>[2x]HHLFKEAQAFIENMYKECHYETQIINKRLHDIELEIKETGTYTHTEEELIYGAKMAWRNSNRCIGRLFWDSLNVIDARDVTDEASFLSSITYHITQATNEGKLKPYITIYAPKDGPKIFNNQLIRYAGYDNCGDPAEKEVTRLANHLGWKGKGTNFDVLPLIYQLPNESVKFYEYPTSLIKEVPIEHNHYPKLRKLNLKWYAVPIISNMDLKIGGIVYPTAPFNGWYMVTEIGVRNFI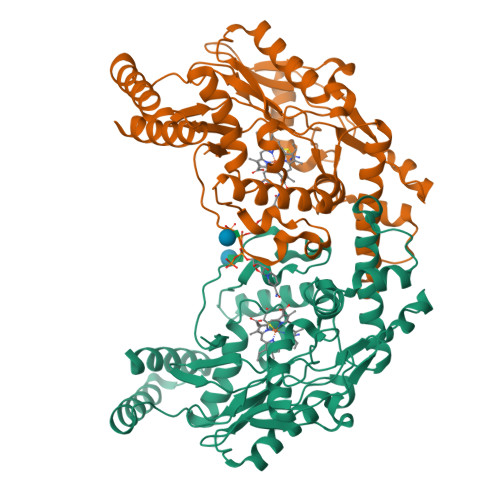DDYRYNLLEKVADAFEFDTLKNNSFNKDRALVELNYAVYHSFKKEGVSIVDHLTAAKQFELFERNEAQQGRQVTGKWSWLAPPLSPTLTSNYHHGYDNTVKDPNFFYKK>GAMEDITSGLKQLDSTYQETNQQVLKNLDEIFSTTSPSANNEMGEEDALNIKKAAIALRGDLALLKANFEANELFFISEDVIFKTYMSSPELLLTYMKINPLDQNTAEQQCGISDKVLVLYCEGKLKIEQEKQNIRERLETSLKAYQSNIGGTASLITASQTLVESLKNKNFIK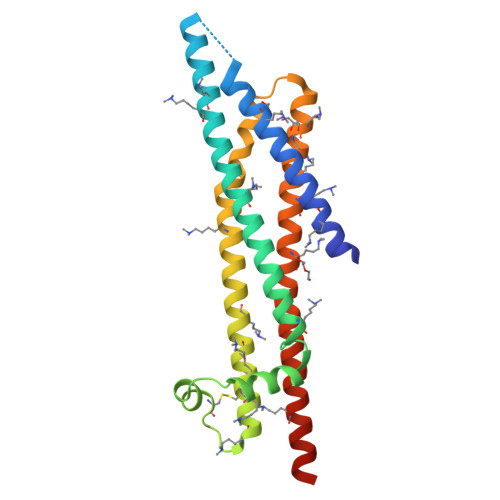GIRKLMLAHNKVFLNYLEELDALERSLEQSKRQYLQERQSSKIIVK[6x]>[4x]SMVKLANPLYTEWILEAIKKVKKQKQRPSEERI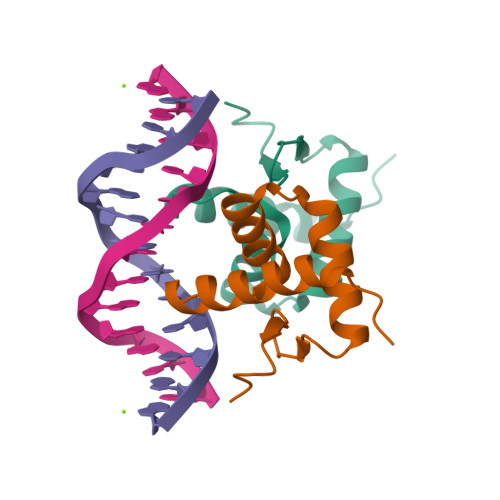CNAVSSSHGLDRKTVLEQLELSVKDGTILKVSNKGLNSYKDPDNPGRIALPKP>GSVGQSLQFLEMGRVTPAQFGAVGDGASHPLSERYATLAEAQTVYPHAVALSDEIDWAALQAAVDSGAPVHIPSGDYQINRGISSTGSLQIAGDGATSIIRPTAAFTGTSVLSCVGSLVALPNISSVSAGSLTIDFASTPNLVAGDVFIIYNPTDSSFSGFRTSYRAGEFCEVRAVSGNTVTIRSALYAAYDGATVAIYKVVSGVVDIASIQIVGGTVPMNGLLVEAVVSPRVDDVTVTLANNAGVYFARCYDAKITNSNISNIGDGGDDYGIIFGNCHDGGADNCKVYARRHAIATGGDAEVGCVPVRNVRMRNCTLRNDITSGTHCADFHGNAEDCSYENCTIYGGATWQGKDISYRHCTITNASGGWIVISAEILGGTFLLDQCTLYTTGDPQPGNRGVIDVGGNSAVLTTNTTQPCNFLIQGGSLRAPSLSTSSYLLRARLEGSTVPVNIQYSGQAIDVGSLGKVLQLDITSGSTSPEYLIVENLAGLPSGITLASAAGGFASAPMRMPVLGGRVQVTTATNASSVTAPVTFRYIYPKAPTVQVTKTDRSYAGNRVGVAIANPTSASGATLGLFTDDGTNFSSAVTNQLNWQAGIYEV[6x]

Bacteriophage-encoded depolymerases are highly specific enzymes, acting at the first step of phage infection and serve for specific recognition of host cell receptor, as well as for the degradation of polysaccharides. The polysaccharide-degrading enzymes are primarily virion-associated proteins like tail fibers, tailspikes, base plate or neck, whereas some are soluble proteins, released during bacterial lysis. These enzymes target structural polysaccharides (LPS, capsular polysaccharides, peptidoglycan) and essential components of the biofilm matrix.

Phage LKA1 encodes a trimeric tailspike protein (LKAgp49) with a typical conserved N-terminal structure-associated domain and an unconserved central and C-terminal region with predicted polysaccharide binding/degrading activity (Pfam 12708 and right-handed β-helices). For crystallization, the N-terminal particle-binding domain of LKAgp49 (residues 1–167) was removed. The resulting mutant – gp49d – constitutes a ‘catalytic module’ of the tailspike. Eventually, one crystal of gp49d gave a clean and isotropic diffraction pattern that extended to 1.9 Å resolution. Gp49d and gp61d display 32% amino acid sequence identity and can be superimposed with a root mean squared deviation of 1.6 Å between 572 (or 97%) equivalent C-alpha atoms. Gp49d can be divided into three domains: (1) a β-helix typical to many tailspikes (residues 181–283 and 371–675); (2) a β-barrel or an insertion domain that is positioned on a side of the β-helix and that interrupts the run of polypeptide chain comprising the β-helix (residues 284–370); and (3) a β-sandwich or jellyroll C-terminal domain (residues 676–769). The most conserved residues form an intricate system connected by hydrogen and ionic bonds with Asp497 coordinating His494 and His499. The three residues are likely to be the most important in the catalysis with Asp497 being the critical residue. A highly conserved Arg329 extends towards the active site where it forms a hydrogen bond with His499. Based on these data, it was concluded that the tailspike protein LKA1gp49 is a specific polysaccharide lyase.>MPAKVLINGYGSIGKRVADAVSMQDDMEVIGVTKTKPDFEARLAVEKGYKLFVAIPDNERVKLFEDAGIPVEGTILDIIEDADIVVDGAPKKIGKQNLENIYKPHKVKAILQGGEKAKDVEDNFNALWSYNRCYGKDYVRVVSCNTTGLCRILYAINSIADIKKARIVLVRRAADPNDDKTGPVNAITPNPVTVPSHHGPDVVSVVPEFEGKILTSAVIVPTTLMHMHTLMVEVDGDVSRDDILEAIKKTPRIITVRAEDGFSSTAKIIEYGRDLGRLRYDINELVVWEESINVLENEIFLMQAVHQESIVIPENIDCIRAMLQMEEDNFKSIEKTNK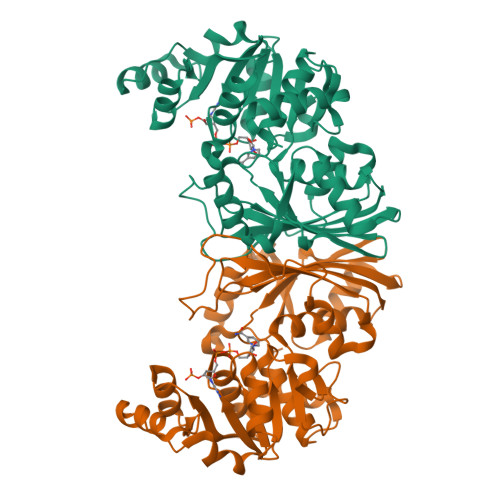AMGIQ[2x]>MSPGERFLDWLKRLQGQKAWTAARAAFRRSLAFPPGAYPRAMPYVEPFLAKGDW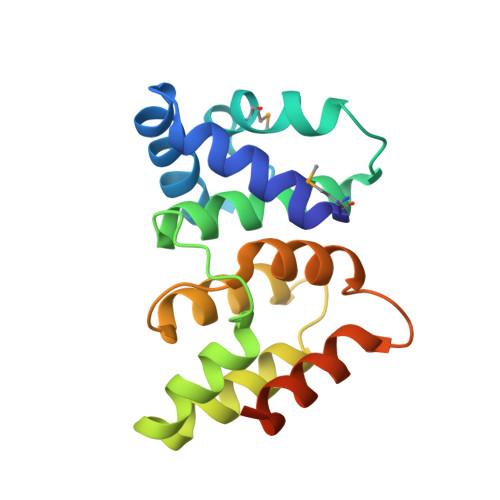RQEEREAHYLVAALYALKDGDHQVGRTLARALWEKAQGSASVEKRFLALLEADRDQIAFRLRQAVALVEGGIDFARLLDDLLRWFSPERHVQARWAREYYGAGASEEEKKKEVEA[2x]> MAQFAFESDLHSLLQLDAPIPNAPPARWQRKAKEAAGPAPSPMRAANRSHSAGRTPGRTPGKSSSKVQTTPSKPGGDRYIPHRSAAQMEVASFLLSKENQPENSQTPTKKEHQKAWALNLNGFDVEEAKILRLSGKPQNAPEGYQNRLKVLYSQKATPGSSRKTCRYIPSLPDRILDAPEIRNDYYLNLVDWSSGNVLAVALDNSVYLWSASSGDILQLLQMEQPGEYISSVAWIKEGNYLAVGTSSAEVQLWDVQQQKRLRNMTSHSARVGSLSWNSYILSSGSRSGHIHHHDVRVAEHHVATLSGHSQEVCGLRWAPDGRHLASGGNDNLVNVWPSAPGEGGWVPLQTFTQHQGAVKAVAWCPWQSNVLATGGGTSDRHIRIWNVCSGACLSAVDAHSQVCSILWSPHYKELISGHGFAQNQLVIWKYPTMAKVAELKGHTSRVLSLTMSPDGATVASAAADETLRLWRCFELDPARRREREKASAAKSSLIHQGIR;> RAPXSDITN

Here we explore peptide inhibitors of Cdc20, a substrate-recognition subunit and activator of the E3 ubiquitin ligase the anaphase-promoting complex/cyclosome (APC/C) that is essential in mitosis and consequently of interest as an anti-cancer target. APC/C engages substrates via degrons that include the ‘destruction box’ (D-box) motif. The D-box binding site comprises a cleft between two of the beta-propeller blades and the neighbouring APC/C subunit APC10, which is thought to result in stabilisation of the active complex. We used a rational design approach to construct binders containing unnatural amino acids aimed at better filling a hydrophobic pocket that contributes to the D-box binding site on the surface of Cdc20.

We incorporated (S)–2-amino-4,4-dimethylpentanoic acid (C3) into the backbone sequences of D4, D10, and D19 replacing leucine at position 4, yielding peptides D7, D12, and D20, respectively. As expected, the structure–activity relationship (SAR) held true between all peptides, whereby incorporation of the unnatural amino acid increased the binding affinity over 6-fold versus the respective parental peptide. Building on this success, we further explored the commercially available halogenated analog, (S)–2-amino-4,4,4-trifluorobutanoic acid (F3), leading to peptide D21. With the tri-fluorinated group, a further increase in binding affinity was achieved (KD = 520 ± 10 nM), which is similar to that of Apcin. We attempted these soaking experiments with our four highest affinity peptides, D21, D20, D7, and D19 (in order of highest affinity to lowest) and were able to observe sufficient ligand density for all but D19. The crystal structures of Cdc20WD40 in complex with each of the other three D-box peptides show that they bound to Cdc20WD40 at the canonical D-box degron binding site, with a largely similar topology to the S. cerevisiae Acm1-Cdh1 structure (overlay of D21 with Acm1 D-box). The guanidino group of the P1 arginine residue of the D-box peptides forms hydrogen bonds with the carboxylate side chains of Asp177 and Glu465 of Cdc20WD40. The nitrogen backbone atom of the (S)–2-amino-4,4,4-trifluorobutanoic acid/(S)–2-amino-4,4-dimethylpentanoic acid unnatural amino acids also forms a hydrogen bond with the carbonyl of Asp177. Additionally, the carbonyl of S5 belonging to D21/D20 forms a H-bond with the nitrogen backbone atom of Asp177. Interestingly, the observed electron density of the peptide correlates with Cdc20 binding affinity: D21 and D20, having the highest affinities, display the clearest electron density allowing six amino acids to be modelled, whereas D7 shows relatively poor density permitting modelling of only four residues.> GSKPHQWQADEEAVRSATCSFSVKYLGCVEVFESRGMQVCEEALKVLRQSRRRPVRGLLHVSGDGLRVVD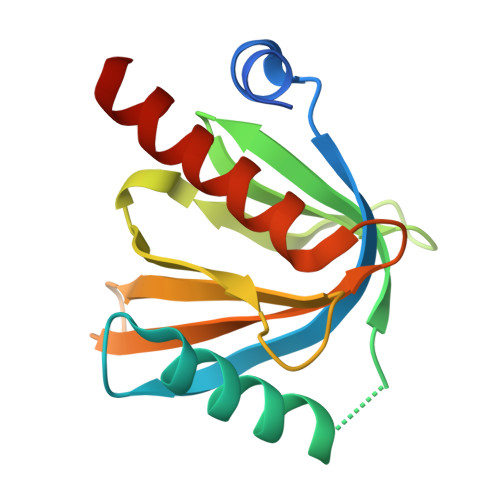DETKGLIVDQTIEKVSFCAPDRNHERGFSYICRDGTTRRWMCHGFLACKDSGERLSHAVGCAFAVCLERKQ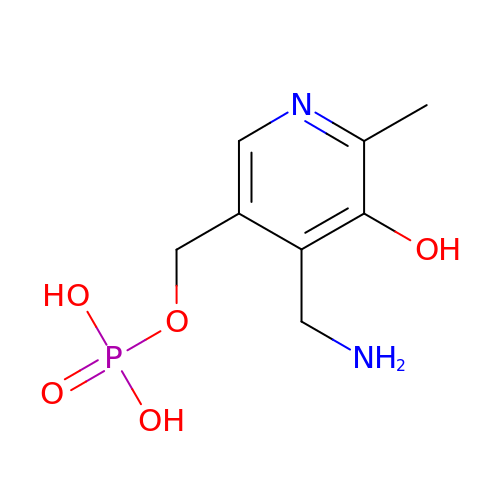4'-DEOXY-4'-AMINOPYRIDOXAL-5'-PHOSPHATE | C8 H13 N2 O5 P | ZMJGSOSNSPKHNH-UHFFFAOYSA-N> KGGAKRH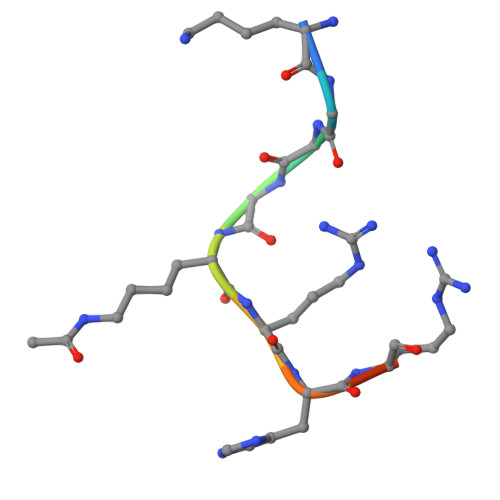RKI> GDVVEAIEGAVARVADTISSGPTNSQAVPALTAVETGHTSQVVPGDTMQTRHVKNYHSRSESTIENFLSRSACVYMGEYYTTNTDETKRFASWTINARRMVQMRRKLEMFTYVRFDVEVTFVITSKQDQGTQLGQDMPPLTHQIMYIPPGGPIPKSTTDYAWQTSTNPSIFWTEGNAPPRMSIPFVSIGNAYSNFYDGWSHFSQNGVYGYNTLNNMGQLYMRHVNGPSPLPMTSIVRVYFKPKHVKAWVPRPPRLCQYKNASTVNFSSTN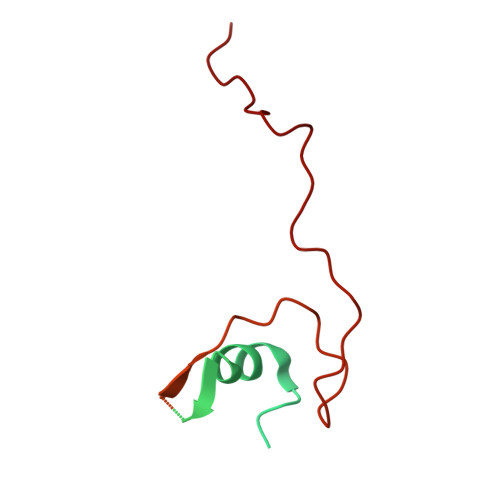ITDKRDSITHVPDTVKP> MATLICGSIAYDNIMTFEGRFREHILPDQVHLINLSFLVPTMRREFGGCAGNIAYALNLLGGDARMMGTLGAVDAQPYLDRMDALGLSREYVRVLPDTYSAQAMITTDLDNNQITAFHPGAMMQSHVNHAGEAKDIKLAIVGPDGFQGMVQHTEELAQAGVPFIFDPGQGLPLFDGATLRRSIELATYIAVN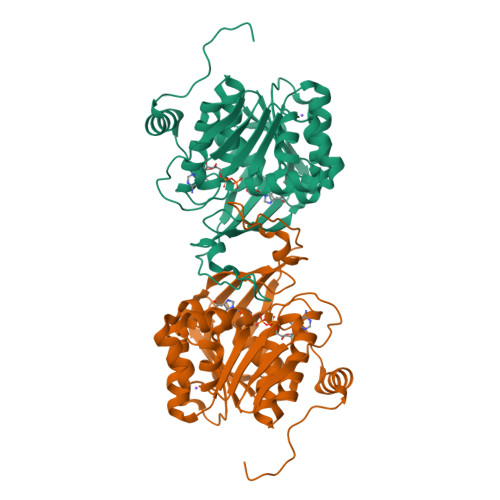DYEAKLVCDKTGWSEDEIASRVQALIITRGEHGATIRHRDGTEQIPAVRAERVIDPTGCGDAFRGGLLYGIEHGFDWATAGRLASLMGALKIAHQGPQTYAPTRAEIDARFETAFGYRPKGSKLRSLEHHHHHH> TQLEEQLHNVETVRSITMQLEMALTKLKKDMMRGGDAKQYQVWQRESKALESAIAIIHYVAGDLK;> SNFSGFTKGTDIADLDAVAQTLKKPADD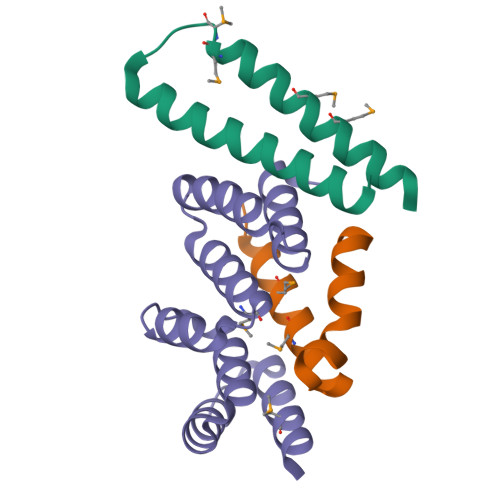ANKAVNDSIAALKDKPDNPALLADLQHSINKWSVIYNINSTIVRSMKDLMQGILQKFP;> SMKYKLNVLLAEIALIGTGNHYHEEANCIAEWLHLKGEEEAVQLIRLSSLMNRGDYASALQQGNKLAYPDLEPWLALCEYRLGLGSALESRLNRLARSQDPRIQTFVNGMREQLKT> GGGGGGGG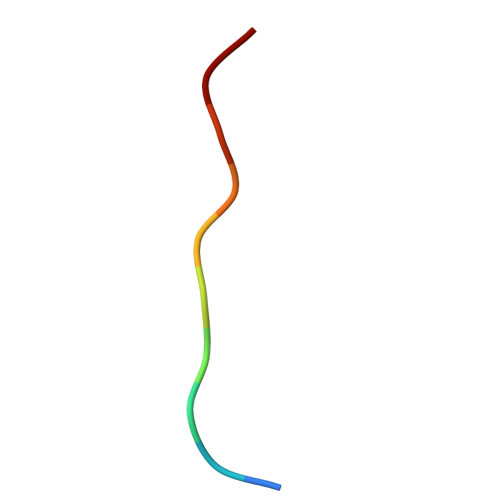GG1-(5-deoxy-5-morpholin-4-yl-alpha-L-arabinofuranosyl)pyrimidine-2,4(1H,3H)-dione | C13 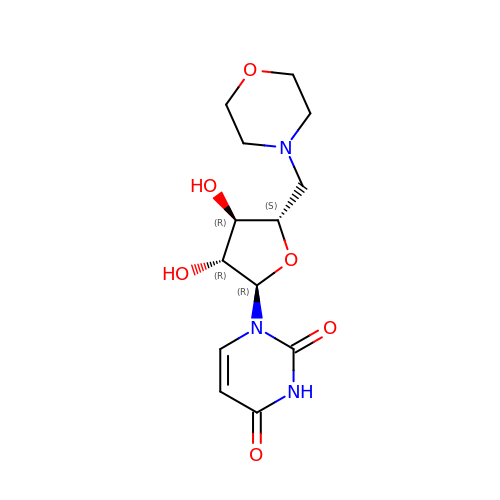H19 N3 O6 | LZYQLCIKQTYBER-OHBODLIOSA-N> MAPHFKEELRNLNVRYQSNATLVCKVTGHPKPIVKWYRQGKEIIADGLKYRIQEFKGGYHQLII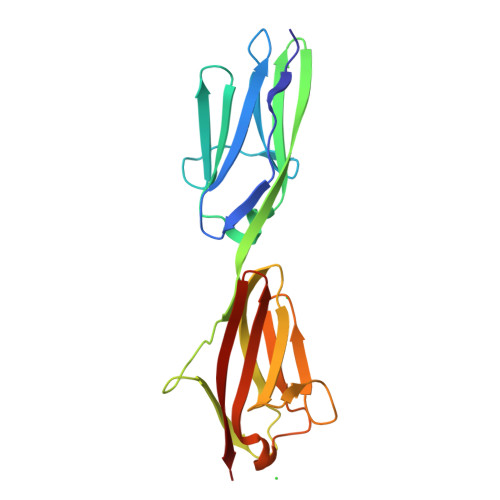ASVTDDDATVYQVRATNQGGSVSGTASLEVEVPAKIHLPKTLEGMGAVHALRGEVVSIKIPFSGKPDPVITWQKGQDLIDNNGHYQVIVTRSFTSLVFPNGVERKDAGFYVVCAKNRFGIDQKTVELDVAD> SAHNAYNAGIMQKTGKAFADEFFAEENQVVHESNAVVLVLMKSDEIDAIIEDIVLKGGKAKNPSIVVEDKAGFWWIKADGAIEIDAAEAGELLGKPFSVYDLLINVASAVGRAYTLGT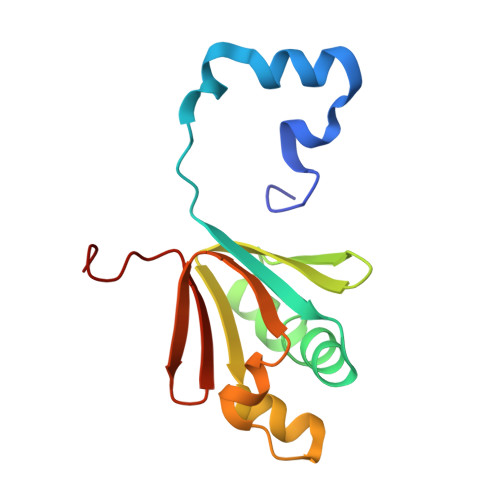KFTITSELMGLDR> GHMIARGKFRSLTLINWNGFFARTFDFDELVTTLSGGNGAGKSTTMA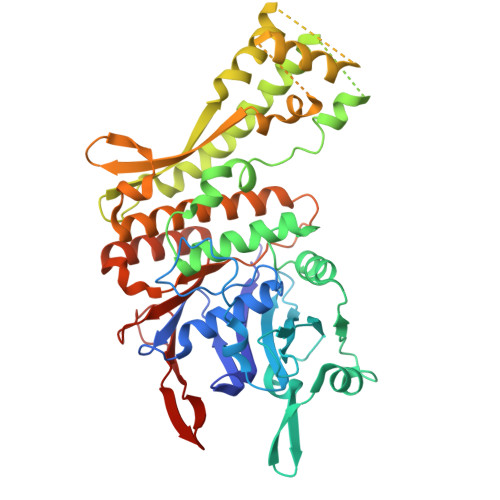GFVTALIPDLTLLNFRNTTEAGSTSSSRDKGLYGKLKAGVCYAVLETVNSRAQRIITGVRLQQIAGRDKKVDIRPFSLQNVPMTDSVISLFTEQVANKARVLSLNDLKEKFEETAVTFKPYHSITDYHSFMFDLGILPKRLRSSSDRNKFYKLIEASLYGGISSVITKSLRDYLLPENSGVRQAFQDMEAALRENSGGSGGSISAESVANILRKTIQREQNRILQLNQGLQNIAFGQVKGVRLVVNIRDTHSILLNALSDQHEQHKDLFESQKLSFSEALAMLYKRINPHIELGQRMPQTIGEELLDYRNYLDLEVETLRGAYGWMRAESSALSTGEAIGTGMSILLMVVQSWEEESRRMRAKDILPCRLLFLDQAARLDAMSINTLFELCERLDMQLLIAAPENISPERGTTYKLVRKILANQEYVHVVGLKGFG KtrAB is a cation channel with a nucleotide-dependent RCK domain. The structure of the KtrAB complex revealed a homodimeric membrane protein (KtrB) assembled with a cytosolic RCK octameric ring, formed by the KtrA protein. KtrA binds nucleotides, ATP or ADP. ATP binding induces the adoption of a square-conformation by the octameric ring and increased K+ flux activity through KtrAB; ADP binding results in a non-square conformation and decreased flux.

We introduced the single-point mutations R16A, R16K, A80P and E125Q in KtrA and tested their impact in the complementation assay. However, and contrary to our predictions, none of the R16 mutations had an impact on the growth phenotype, while E125Q resulted in an apparently inactive KtrAB. Crystal structures of the mutants that did not rescue the TK2420 growth phenotype (A80P and E125Q) reveal a different picture. The ATP-bound structures do not adopt a square conformation, displaying L1/L2 distances for A80P (at 3.9 Å resolution) of 52/23 Å and for E125Q (at 4.1 Å resolution and with two different half-rings in the asymmetric unit) of 34/30 Å and 42/27 Å. In contrast, mutants that do not rescue growth (A80P and E125Q) also do not adopt the square conformation in the ATP-bound structures. In contrast, in the maps for the E125Q-ATP structure we do not observe obvious changes in the main-chain trace that might explain the impact of the mutation in the conformation of the ring. Overall, these structural results reveal that E125 coordinates Mg2+ at the intra-dimer interface. Mutation to glutamine likely affects the coordination of the Mg2+ binding site, changing the stability of the square conformation and explaining the inability of the E125Q KtrA mutant to rescue the TK2420 phenotype. Next, we removed the chemical groups that coordinate Mg2+ in the R16K and WT-ATP structures by substituting ATP for ADP or mutating E125 to a glutamine and measured flux. Relative to KtrAB-ATP with Mg2+, flux was 14-fold and 24-fold slower for KtrAB-ADP and KtrAE125QB-ATP with Mg2+, respectively (Figure 6c and Figure 6—source data 1). To explore the possibility that choline is an activator we analyzed the impact of the E125Q mutation and of ADP in the presence of 150 mM choline. Both KtrAE125QB-ATP and KtrAB-ADP display low ion flux, with rates that are 12- and 16-fold slower than for KtrAB-ATP (Figure 8b and c and Figure 8—source data 1).

>[8x]MGRIKNKQFAVIGLGRFGGSICKELHRMGHEVLAVDINEEKVNAYASYATHAVIANATEENELLSLGIRNFEYVIVAIGANIQASTLTTLLLKELDIPNIWVKAQNYYHHKVLEKIGADRIIHPQKDMGVKIAQSLSDENVLNYIDLSDEYSIVELLATRKLDSKSIIDLNVRAKYGCTILAIKHHGDICLSPAPEDIIREQDCLVIMGHKKDIKRFENEGM>[4x]MDYKDDDDKLEMPMAQSSCPGSPPDTGDGWEPVLCKGEVNFGGSGKKRSKFVKVPSNVAPSMLFELLLTEWHLPAPNLVVSLVGEERLFAMKSWLRDVLRKGLVKAAQSTGAWILTSALHVGLARHVGQAVRDHSLASTSTKVRVVAIGMASLDRILHRQLLDGVQAQEDTPIHYPADEGSTQGPLCPLDSNLSHFILVEPGTLGSGNDGLAELQLSLEKHISQQRTGYGGTSSIQIPVLCLLVNGDPSTLERMSRAVEQAAPWLILAGSGGIADVLAALVGQPHLLVPQVTEKQFREKFPSECFSWEAIVHWTELLQNIAAHPHLLTVYDFEQEGSEDLDTVILKALVKACKSHSRDAQDYLDELKLAVAWDRVDIAKSEIFNGDVEWKSCDLEEVMTDALVSNKPDFVRLFVDSGADMAEFLTYGRLQQLYHSVSPKSLLFELLERKHEEGRLTLAGLGAQQTRELPVGLPAFSLHEVSRVLKDFLHDACRGFYQDGRRMEERGPPKRPAGQKWLPDLSRKSEDPWRDLFLWAVLQNRYEMATYFWAMGRE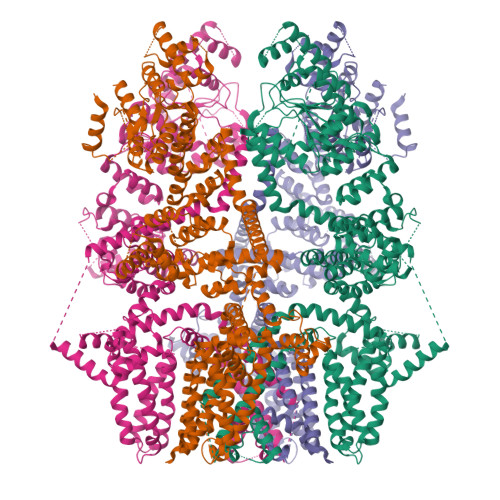GVAAALAACKIIKEMSHLEKEAEVARTMREAKYEQLALDLFSECYSNSEDRAFALLVRRNHSWSRTTCLHLATEADAKAFFAHDGVQAFLTKIWWGDMATGTPILRLLGAFTCPALIYTNLISFSEDAPQRMDLEDLQEPDSLDMEKSFLCSHGGQLEKLTEAPRAPGDLGPQAAFLLTRWRKFWGAPVTVFLGNVVMYFAFLFLFSYVLLVDFRPPPQGPSGSEVTLYFWVFTLVLEEIRQGFFTNEDTRLVKKFTLYVEDNWNKCDMVAIFLFIVGVTCRMVPSVFEAGRTVLAIDFMVFTLRLIHIFAIHKQLGPKIIIVERMMKDVFFFLFFLSVWLVAYGVTTQALLHPHDGRLEWIFRRVLYRPYLQIFGQIPLDEIDEARVNCSLHPLLLDSSASCPNLYANWLVILLLVTFLLVTNVLLMNLLIAMFSYTFQVVQGNADMFWKFQRYHLIVEYHGRPALAPPFILLSHLSLVLKQVFRKEAQHKQQHLERDLPDPVDQKIITWETVQKENFLSTMEKRRRDSEEEVLRKTAHRVDLIAKYIGGLREQEKRIKCLESQANYCMLLLSSMTDTLAPGGTYSSSQNCGRRSQPASARDREYLEAGLPHSDT5-AMINO-1H-PYRIMIDINE-2,4-DIONE 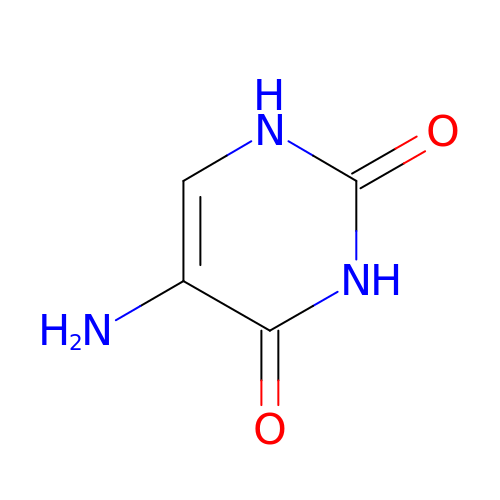| C4 H5 N3 O2 | BISHACNKZIBDFM-UHFFFAOYSA-N>[2x]QEQVAPPKDPAAALEDHKTRTDNRYEPSLDNLAQQDVAAPGAPEGVTALSDAQYNEANKIYFERCAGCHGVLRKGATGKALTPDLTRDLGFDYLQSFITYASPAGMPNWGTSGELSAEQVDLMANYLLLDPAAPPEFGMKEMRESWKVHVAPEDRPTQQMNDWDLENLFSVTLRDAGQIALIDGSTYEIKTVLDTGYAVHISRLSASGRYLFVIGRDGKVNMIDLWMKEPTTVAEIKIGSEARSIETSKMEGWEDKYAIAGAYWPPQYVIMDGETLEPKKIQSTRGMTYDEQEYHPEPRVAAILASHYRPEFIVNVKETGKILLVDYTDLNNLKTTEISAERFLHDGGLDGSHRYFITAANARNKLVVIDTKEGKLVAIEDTGGQTPHPGRGANFVHPTFGPVWATSHMGDDSVALIGTDPEGHPDNAW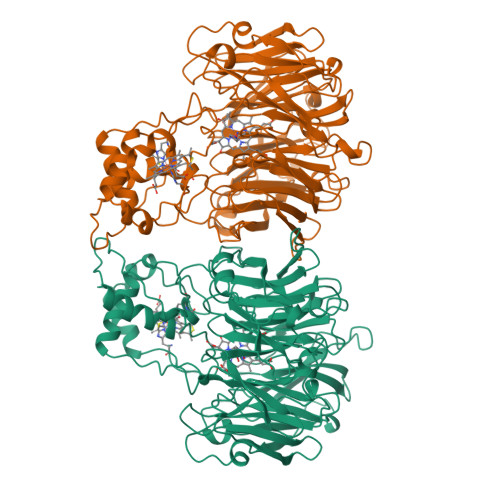KILDSFPALGGGSLFIKTHPNSQYLYVDATLNPEAEISGSVAVFDIKAMTGDGSDPEFKTLPIAEWAGITEGQPRVVQGEFNKDGTEVWFSVWNGKDQESALVVVDDKTLELKHVIKDERLVTPTGKFNVYNTMTDTY> 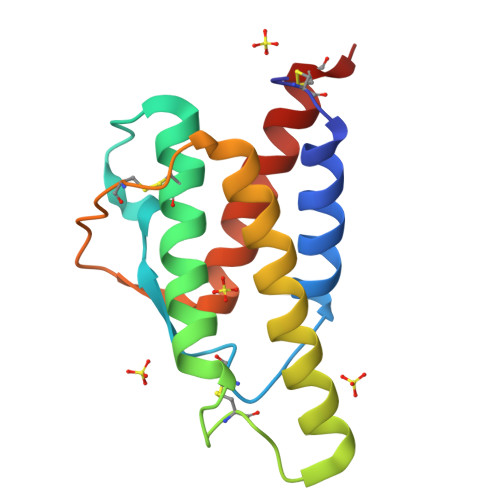HKCDITLQEIIKTLNSLTEQKTLCTELTVTDIFAASKNTTEKETFCRAATVLRQFYSHHEKDTRCLGATAQQFHRHKQLIRFLKALDRNLWGLAGLNSCPVKEANQSTLENFLERLKTIMREKYSKCSS>MAVEPFPRRPITRPHASIEVDTSGIGGSAGSSEKVFCLIGQAEGGEPNTVYELRNYSQAKRLFRSGELLDAIELAWGSNPNYTAGRILAMRIEDAKPASAEIGGLKITSKIYGNVANNIQVGLEKNTLSDSLRLRVIFQDDRFNEVYDNIGNIFTIKYKGEEANATFSVEHDEETQKASRLVLKVGDQEVKSYDLTGGAYDYTNAIITDINQLPDFEAKLSPFGDKNLESSKLDKIENANIKDKAVYVKAVFGDLEKQTAYNGIVSFEQLNAEGEVPSNVEVEAGEESATVTATSPIKTIEPFELTKLKGGTNGEPPATWADKLDKFAHEGGYYIVPLSSKQSVHAEVASFVKERSDAGEPMRAIVGGGFNESKEQLFGRQASLSNPRVSLVANSGTFVMDDGRKNHVPAYMVAVALGGLASGLEIGESITFKPLRVSSLDQIYESIDLDELNENGIISIEFVRNRTNTFFRIVDDVTTFNDKSDPVKAEMAVGEANDFLVSELKVQLEDQFIGTRTINTSASIIKDFIQSYLGRKKRDNEIQDFPAEDVQVIVEGNEARISMTVYPIRSFKKISVSLVYKQQTLQA[3x];> MAITSVDSYLLSEIKPRLNTVLENCYIIDEVLKDFDYQTRESFKEAFCGKNAQHEVTVGFNFPKFKNNYEAHYLIQLGQGQETKNSLGSIQSSYFEATGDTLVESSTAIREDDKLVFTVSKPIGELIKVEDIEFAKYDNLQVEGNKVSFKYQTNEDYENYNANIIFTEKKNDSKGLVKGFTVE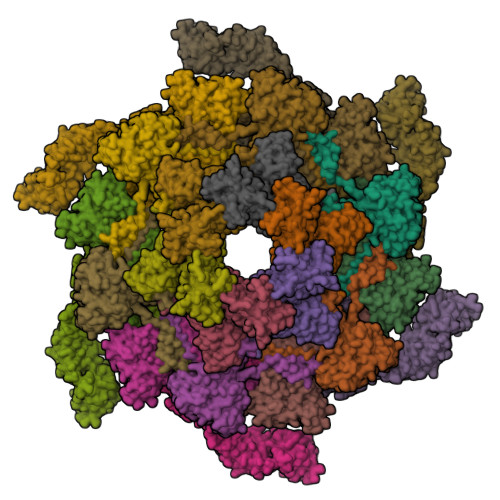EQVTVVGLSFNVDVARCLDAVLKMILISMRDSIEEQQTFQLQNLSFGDIAPIIEDGDSMIFGRPTIIKYTSSLDLDYTITQDINKLTFKERKDWK>SWVQLAGHTGSFKAAGTSGLILKRSSEPEHYCMVRLMADVLRGCVPAFHGVVERDGESYLQLQDLLDGFDGPCVLDCKMGVRTYLEEELTKARERPKLRKDMYKKMLAVDPEAPTEEEHAQRAVTKPRYMQWREGISSSTTLGFRIEGIKKADGSCSTDFKTTRSREQVTRVFEEFMQGDAEVLKRYLNRLQQIRDTLEISDFFRRHEVIGSSLLFVHDHCHRAGVWLIDFGKTTPLPNGQILDHRRPWEEGNREDGYLLGLDNLIGILANLAE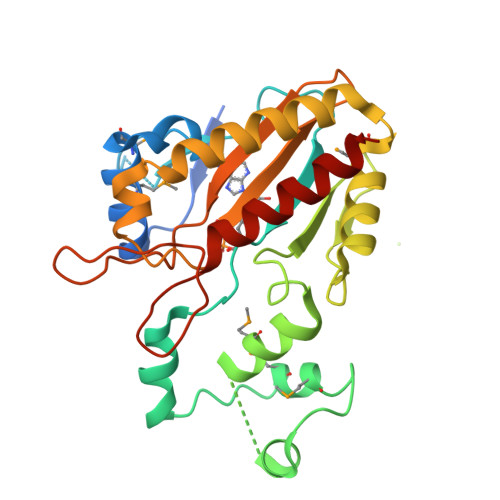R[2x]>MEKAHPKEMVPLMGKRVAAPSGNPAILPEKRPAEITPTKKSAHFFLEIEGFEPNPTVAKTSPPVFSKPMDSNIRQCISGNCDDMDSPQSPQDDVTETPSNPNSPSAQLAKEEQRRKKRRLKKRIFAAVSEGCVEELVELLVELQELCRRRHDEDVPDFLMHKLTASDTGKTCLMKALLNINPNTKEIVRILLAFAEENDILGRFINAEYTEEAYEGQTALNIAIERRQGDIAALLIAAGADVNAHAKGAFFNPKYQHEGFYFGETPLALAACTNQPEIVQLLMEHEQTDITSRDSRGNNILHALVTVAEDFKTQNDFVKRMYDMILLRSGNWELETTRNNDGLTPLQLAAKMGKAEILKYILSREIKEKRLRSLSRKFTDWAYGPVSSSLYDLTNVDTTTDNSVLEITVYNTNIDNRHEMLTLEPLHTLLHMKWKKFAKHMFFLSFCFYFFYNITLTLVSYYRPREEEAIPHPLALTHKMGWLQLLGRMFVLIWAMCISVKEGIAIFLLRPSDLQSILSDAWFHFVFFIQAVLVILSVFLYLFAYKEYLACLVLAMALGWANMLYYTRGFQSMGMYSVMIQKVILHDVLKFLFVYIVFL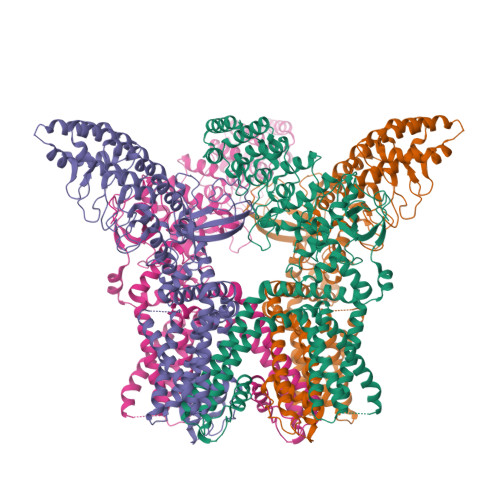LGFGVALASLIEKCPKDNKDCSSYGSFSDAVLELFKLTIGLGDLNIQQNSKYPILFLFLLITYVILTFVLLLNMLIALMGETVENVSKESERIWRLQRARTILEFEKMLPEWLRSRFRMGELCKVAEDDFRLCLRINEVKWTEWKTHVSFLNEDPGPVRRTDFNKIQDSSRNNSKTTLNAFEEVEEFPETSVVDAGLEVLFQGPAAAVDYKDDDDKAHHHHHHHHHH[4x]Here, we report crystallographic and biochemical results on the structure and substrate selectivity of AspH. The results reveal a key role for the TPR domain of AspH in substrate binding and, unexpectedly, that the preferred EGFD-substrates of AspH have a non-canonical (Cys3–4) disulfide pattern. Whilst the oxygenase domain fold of AspH is typical for the 2OG oxygenase superfamily, details of its active site and the role of the TPR domain in EGFD-substrate binding are remarkable. Whatever the precise extent of conformational changes during catalysis, the results reveal a central role for the TPR domain in enabling AspH catalysis—without it, 2OG turnover occurs, but EGFDs are not hydroxylated.

Next, we assayed AspH for its ability to hydroxylate truncated 26mer hFX EGF1 substrates (aa 86–111) lacking the Cys5–6 disulfide-forming residues, synthesized using orthogonal cysteine protection to yield selectively both the pure canonical (C26mer) or non-canonical (NC26mer) disulfide isomers. Only the NC26mer peptide was hydroxylated under normal assay conditions, whereas both 26mer peptides were hydroxylated using redox buffer conditions. A structure of AspH in complex with NC26mer was obtained (AspH-TPR-Ox:NC26mer). Comparison of AspH-TPR-Ox:NC26mer and AspH-TPR-Ox:hFX structures reveals little overall difference (Cα RMSD 0.13 Å). The presence of a Cys3–4 disulfide bond indicates that the additional residues present in the longer 39mer substrate, which were not observed in electron density maps of AspH-TPR-Ox:NC26mer due to disorder, are likely not essential for substrate recognition.

> KPKLLNKFDKTIKAELDAAEKLRKRGKIEEAVNAFKELVRKYPQSPRARYGKAQCEDDLAEKRRSNEVLRGAIETYQEVASLPDVPADLLKLSLKRRSDRQQFLGHMRGSLLTLQRLVQLFPNDTSLKNDLGVGYLLIGDNDNAKKVYEEVLSVTPNDGFAKVHYGFILKAQNKIAESIPYLKEGIESGDPGTDDGRFYFHLGDAMQRVGNKEAYKWYELGHKRGHFASVWQRSLYNVNGLKAQPWWTPKETGYTELVKSLERNWKLIRDEGLAVMDKAKGLFLPEDENLREKGDWSQFTLWQQGRRNENACKGAPKTCTLLEKFPETTGCRRGQIKYSIMHPGTHVWPHTGPTNCRLRMHLGLVIPKEGCKIRCANETKTWEEGKVLIFDDSFEHEVWQDASSFRLIFIVDVWHPELTPQQRRSLPAI;> DGDQCETSPCQNQGKCKDGLGEYTCT(2S)-pentane-1,2-diol | C5 H12 O2 | 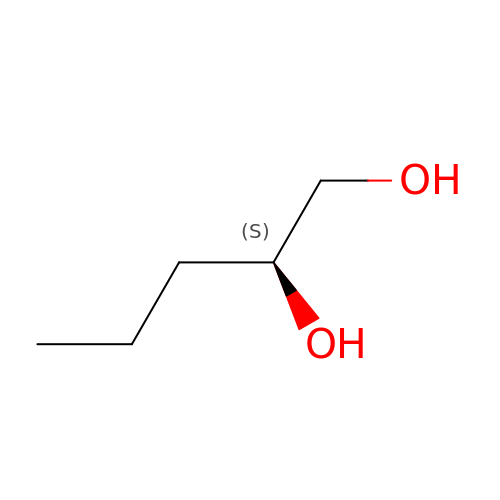WCVRQHFDJLLWFE-YFKPBYRVSA-N> NFTAPVTTPSIPTPIQFLQTWLPGFVKVMTAARKIDEIIGIDTVGSWEDQEIVQGIVEPAGTAVEYGDHTNIPLTSWNANFERRTIVRGELGMMVGTLEEGRASAIRLNSAETKRQQ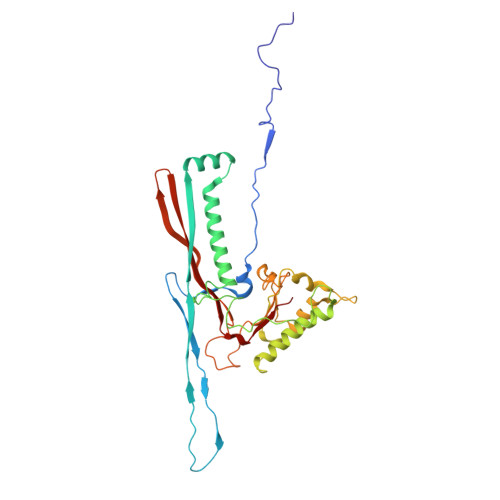AAIGLETFRNAIGFYGWQSGLGNRTYGFLNDPNLPAFQTPPSQGWSTADWAGIIGDIREAVRQLRIQSQDQIDPKAEKITLALATSKVDYLSVTTPYGISVSDWIEQTYPKMRIVSAPELSGVQMKNQEPEDALVLFVEDVNAAVDGSTDGGSVFSQLVQSKFITLGVEKRAKSYVEDFSNGTAGALCKRPWAVVRYLGI1-({4-[(3-aminopropyl)amino]butyl}amino)ethane-1,1-diol 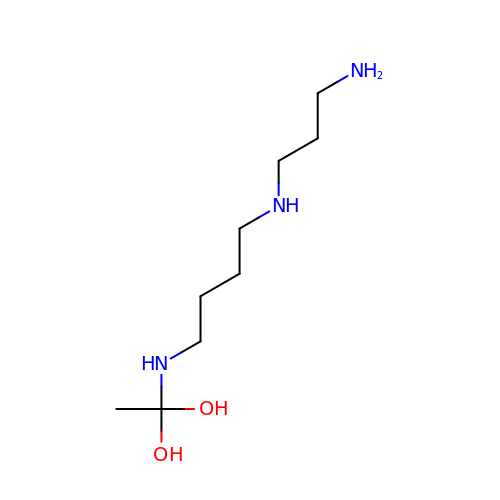| C9 H23 N3 O2 | WAYWJVQKELFVTE-UHFFFAOYSA-N>GAASMNAAVVRRTQEALGKVIRRPPLTEKLLNKPPFRYLHDIITEVIRITGFMKGLYTDAEMKSENVKDKDAKIS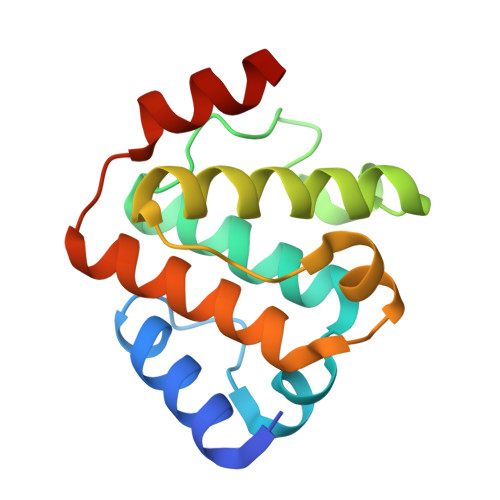FLQKAIDVVMMVSGEPLAAKPARIVAGHEPERTNELLQLIGKCCLSKLSSDEAVKRVLAGDK[4x]2-methyl-1,3-thiazole-5-carboxylic acid | C5 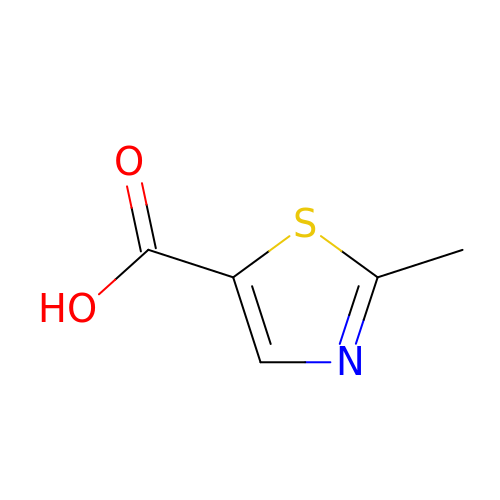H5 N O2 S | QCXCIYPOMMIBHO-UHFFFAOYSA-N>[2x]XSLSDKDKAAVRALWSKIGKSSDAIGNDALSRMIVVYPQTKIYFSHWPDVTPGSPNIKAHGKKVMGGIALAVSKIDDLK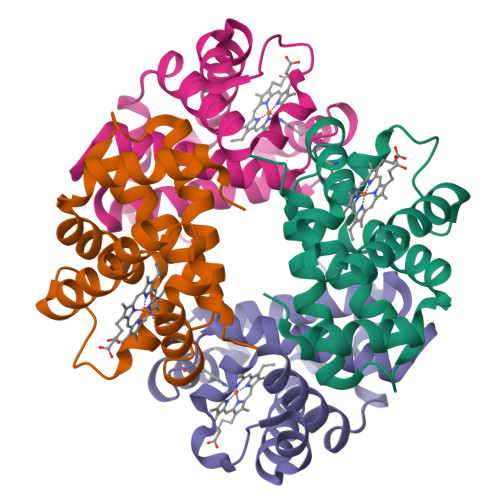TGLMELSEQHAYKLRVDPSNFKILNHCILVVISTMFPKEFTPEAHVSLDKFLSGVALALAERYR;>VEWTDFERATIKDIFSKLEYDVVGPATLARCLVVYPWTQRYFGKFGNLYNAAAIAQNAMVSKHGTTILNGLDRAVKNMDDITNTYAELSVLHSEKLHVDPDNFKLLADCLTIVVAARFGSAFTGEVQAAFQKFMAVVVSSLGKQYR[2x]> EVCSEQAETGPCKAMISRWYFDVTEGKCAPFFYGGCGGNR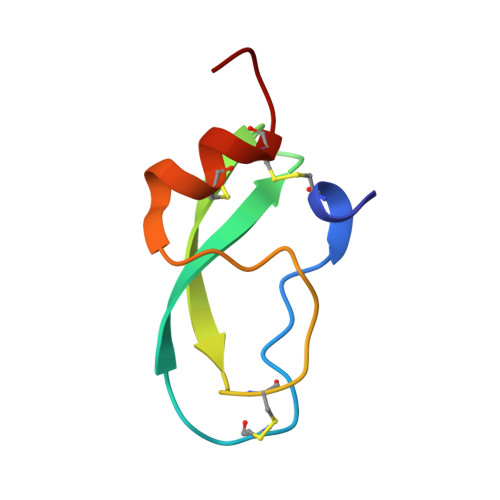NNFDTEEYCMAVCGSAI> DREKIYQWINELSSPETRENALLELSKKRESVPDLAPM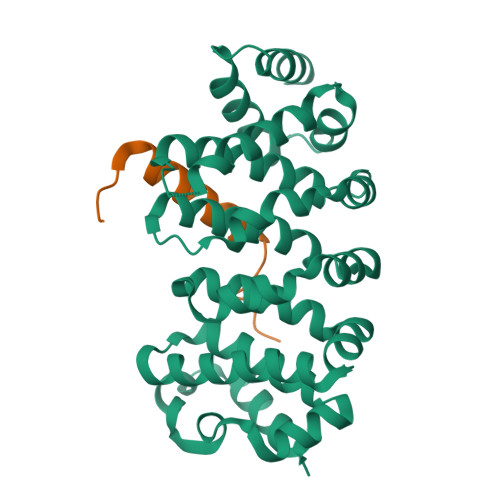LWHSFGTIAALLQEIVNIYPSINPPTLTAHQSNRVCNALALLQCVASHPETRSAFLAAHIPLFLYPFLHTVSKTRPFEYLRLTSLGVIGALVKTDEQEVINFLLTTEIIPLCLRIMESGSELSKTVATFILQKILLDDTGLAYICQTYERFSHVAMILGKMVLQLSKEPSARLLKHVVRCYLRLSDNPRAREALRQCLPDQLKDTTFAQVLKDDTTTKRWLAQLVKNLQ;> HMWETLDDQRALQLALDQLSLLGLDSDE(2S,3R)-2-amino-9-methoxy-3-(2,4,5-trifluorophenyl)-2,3-dihydro-1H-naphtho[2,1-b]pyran-8-carbonitrile 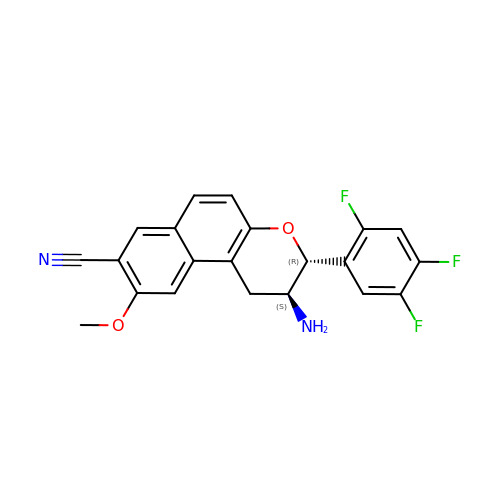| C21 H15 F3 N2 O2 | OGGAKUIGELBYAA-GHTZIAJQSA-N>KDSLRPKLSEEQQHIIAILLDAHHKTYDPTYADFRDFRPPVRMDGS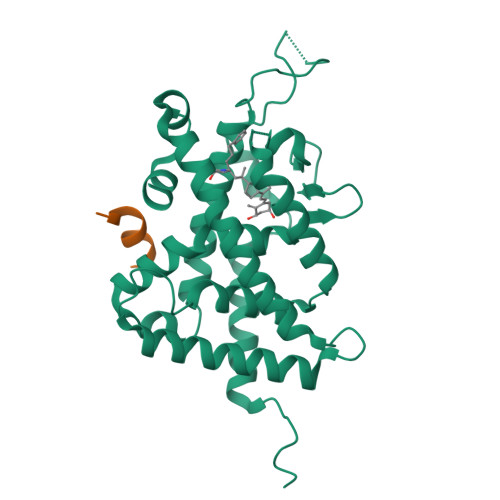TGSVTLDLSPLSMLPHLADLVSYSIQKVIGFAKMIPGFRDLTSDDQIVLLKSSAIEVIMLRSNQSFTMDDMSWDCGSQDYKYDVTDVSKAGHTLELIEPLIKFQVGLKKLNLHEEEHVLLMAICIVSPDRPGVQDAKLVEAIQDRLSNTLQTYIRCRHPPPGSHQLYAKMIQKLADLRSLNEEHSKQYRSLSFQPENSMKLTPLVLEVFG[2x];>NHPMLMNLLK[2x]> DQTVSDNELQEMSNQGSKYVNKEIQNAVNGVKQIKTLIEKTNEERKTLLSNLEEAKKKKEDALNETRESETKLKELPGVCNETMMALWEECKPCLKQTCMKFYARVCRSGSGLVGRQLEEFLNQSSPFYFWMNGDRIDSLLENDRQQTHMLDVMQDHFSRASSIIDELFQDRFFTREPQDTYHYLPFSLPHNFHAMFQPFLEMIHEAQQAMDIHFHSPAFQHPPTEFIREGDDDRTVCREIRHNSTGCLRMKDQCDKCREILSVDCSTNNPSQAKLRRELDESLQVAERLTRKYNELLKSYQWKMLNTSSLLEQLNEQFNWVSRLANLTQGEDQYYLRVTTVASHTSDSDVPSGVTEVVVKLFDSDPITVTVPVEVSRKNPKFMETVAEKALQEYRKKHREE

Clusterin (apolipoprotein J), a conserved glycoprotein abundant in blood and cerebrospinal fluid, functions as a molecular chaperone and apolipoprotein. The Clu structure is composed of three domains, a coiled-coil (CC) domain, a small helical domain containing all disulfide bridges (hereafter disulfide domain, DD) and a C-terminal α/β roll-like (AB) domain. Structure-based mutational analysis demonstrated that two disordered, hydrophobic peptide tails enable diverse activities. Resembling the substrate-binding regions of small heat-shock proteins, these sequences mediate clusterin’s chaperone function in suppressing amyloid-β, tau and α-synuclein aggregation.

For crystallization, we designed a single-chain construct (Clu-Δ(214–238)) comprising a deletion of a predicted unstructured sequence including the furin cleavage site. Upon expression in the presence of the α-mannosidase I inhibitor kifunensine to generate uniform oligomannose N-glycans, purified Clu-Δ(214–238) crystallized at acidic pH in two distinct lattice types, crystal forms I and II, diffracting to 2.8-Å and 3.5-Å resolution, respectively. Crystal form I contained one copy of Clu-Δ(214–238) while crystal form II contained two independent copies. The asymmetric unit of crystal form I is shown in orthogonal views. The dashed line indicates a disordered loop, residues 261–280. The α7–α8 loop (residues 261–280) is also disordered. The three conformations in the crystal lattices differed slightly in their domain orientations, with root-mean-square deviation (r.m.s.d.) values of 1.5–2.0 Å (Cα positions). While the DD seems fairly rigid, its linkers to helices α2 and α10 deviate considerably between crystal forms, indicating structural plasticity. The N-glycans in Clu-Δ(214–238) point toward solvent channels in the crystal lattices and are partially ordered (gray spheres). Importantly, the model of the WT structure contains extended unstructured regions, including disordered tails at the C terminus of the β-chain (residues 199–227) and at the N terminus of the α-chain (residues 228–244). These tails are generated by furin cleavage in the unstructured sequence of WT Clu that is deleted in Clu-Δ(214–238).>[2x]MGKYFG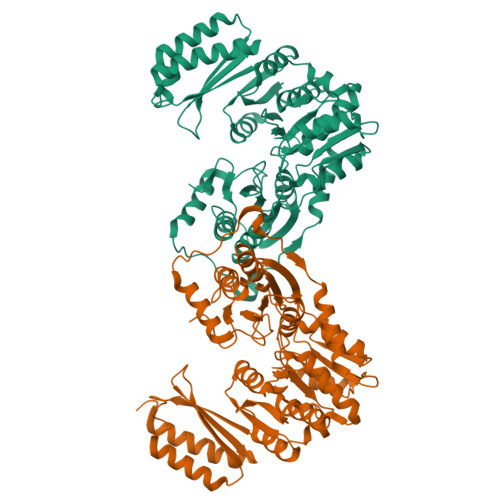TDGVRGVANQELTPELAFKLGRYGGYVLAHNKGEKHPRVLVGRDTRVSGEMLESALIAGLISIGAEVMRLGIISTPGVAYLTRDMGAELGVMISASHNPVADNGIKFFGSDGFKLSDEQENEIEALLDQENPELPRPVGNDIVHYSDYFEGAQKYLSYLKSTVDVNFEGLKIALDGANGSTSSLAPFLFGDLEADTETIGCSPDGYNINEKCGSTHPEKLAEKVVETESDFGLAFDGDGDRIIAVDENGQIVDGDQIMFIIGQEMHKNQELNNDMIVSTVMSNLGFYKALEQEGIKSNKTKVGDRYVVEEMRRGNYNLGGEQSGHIVMMDYNTTGDGLLTGIQLASVIKMTGKSLSELAGQMKKYPQSLINVRVTDKYRVEENVDVKEVMTKVEVEMNGEGRILVRPSGTEPLVRVMVEAATDEDAERFAQQIADVVQDKMGLDKLVPR> MAFKVISQENLLEQKRKETLQEDIPFIVNGEMEYVTKKISNGEMETLE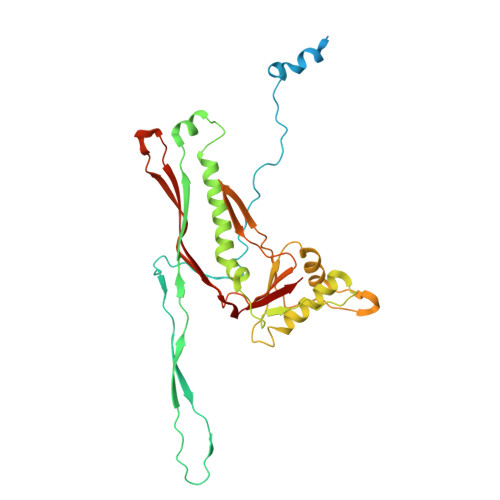LNKPLGEMMTFSSTSNLKELLRKVVLDVELGREQVQLLYKPIYDSIADSNLPQVMDAKWALQGNCVFLEHIEGEEIKFGTINAENGPVARIQTYATGFEYTKEMKDFNQTFSVEILNKSIGESYNALLNHIHLSPIINFNYKASNKTAFKGETNDPIWLGIWRTLTQAQKDTVIAKRQGNILMASSADQIEIEMALNGGHLLNGSMYPSIKNISTVIYYDGWEVTVGKKTYSYKGVTPGKGYLIRPKRGFKELIKRDLTTEVGNADLSKLVENQIVGHCYRGAFAAVEENVQEISFR> TGLHFGRLSLRSLTAYAPNLMLWGGASMLGLFVFTEG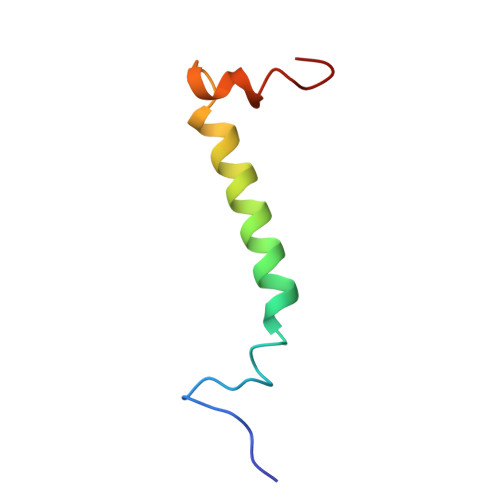WPKFQDTLYKKIPL> GSHMAVQIGFLLFPEVQQLDLTGPHDVLASLPDVQVHLIWKEPGPVVASSGLVLQATTSFADCPP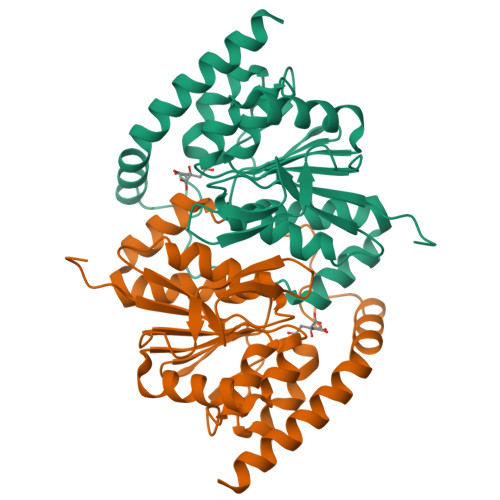LDVICIPGGTGVGALMEDPQALAFIRQQAARARYVTSVCSGSLVLGAAGLLQGKRATTHWAYHELLAPLGAIPVHERVVRDGNLLTGGGITAGIDFALTLAAELFDAATAQRVQLQLEYAPAPPFNAGSPDTAPASVVQQARQRAADSLHKRREITLRAAARLAAG> MTTLTRQDLNSAQVVADVLSEFLEVAVHLILYVREVYPVGIFQKRKKYNVPVQMSCHPELNQYIQDTLHCVKPLLEKNDVEKVVVVILDKEHRPVEKFVFEITQPPLLSINSDSLLSHVEQLLRAFILKISKVDK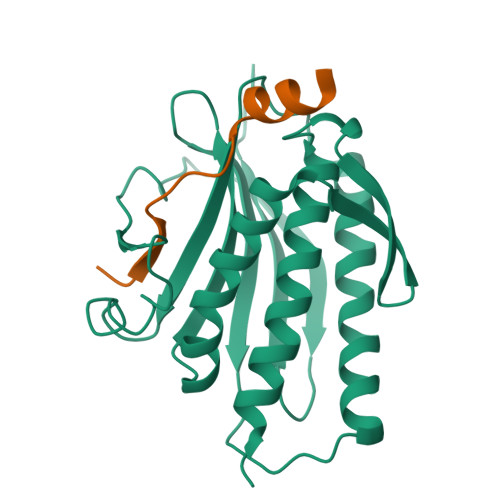VLDHNPPGCTFTVLVHTREAATRNMEKIQVIKDFPWILADEQDVHMHDPRLIPLKTMTSDILKMQLYVEERAHKNS;> MGRTANILKPLMSPPSREEIMATLLDHD> MPSYKSSRVLVRDVPEELVDHYERSHRVAAFFMRLLLAMRREPYSLRMRDGTEREVDLDETDDFLRSAGCEEPDAVSDDLRSFALAVLHQDNPKKRAFLESENCVSILCLEKSASGTRYYKRPGYQLLKKAIEEEWGWDKFEASLLDERTGEVAEKFAALSMEDWRRFFAARDPDDLGRELLKTDTREGMAAALRLRERGVFPVSVPEHLDLDSLKAAMASAAERLKSWLACNQRAVDEKSELRKRFEEALDGVDPEKYALFEKFAAELQQADYNVTKKLVLAVSAKFPATEPSEFKRGVEILKEDGYKPLWEDFRELGFVYLAERKWERRRGGAAVTLCDADDSPIKVRFGLTGRGRKFVLSAAGSRFLITVKLPCGD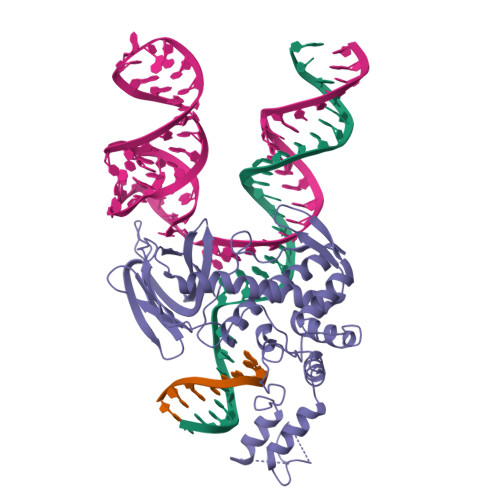VGLTAVPSRYFWNPSVGRTTSNSFRIEFTKRTTENRRYVGEVKEIGLVRQRGRYYFFIDYNFDPE>NTTQQGSPVFAKLLAKNQASLCNTTLNWHSQDGAGSSYLSQGLRYEEDKKELVVDSPGLYYVFLELKLSPTFTNTGHKVQGWVSLVLQAKPQVDDFDNLALTVELFPCSMENKLVDRSWSQLLLLKAGHRLSVGLRAYLHGAQDAYRDWELSYPNTTSFGLFLVKPDNPWE[2x];>DPVQNSCDNCQPGTFCRKYNPVCKSCPPSTFSSIGGQPNCNICRVCAGYFRFKKFCSSTHNAECECIEGFHCLGPQCTRCEKDCRPGQELTKQGCKTCS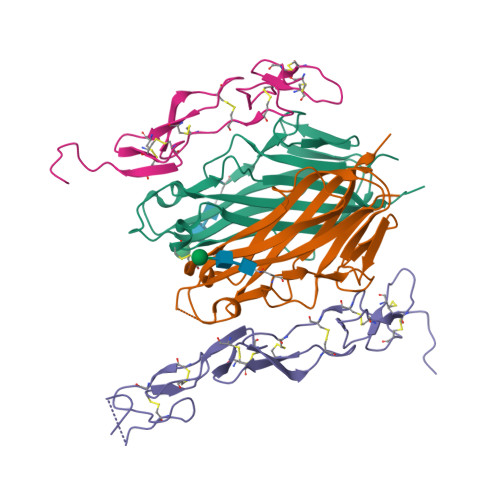LGTFNDQNGTGVCRPWTNCSLDGRSVLKTGTTEKDVVCGP[2x]>MGDCDIEGKDGKQYESVLMVSIDQLLDSMKEIGSNCLNNEFNFFKRHICDANKE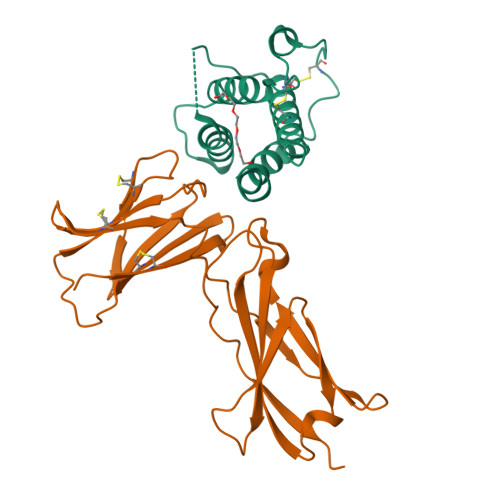GMFLFRAARKLRQFLKMNSTGDFDLHLLKVSEGTTILLNCTGQVKGRKPAALGAAQPTKSLEENKSLKEQKKLNDLCFLKRLLQEIKTCWNKILMGTKEH[2x];>GSHMESGYAQNGDLEDAELDDYSFSCYSQLEVNGSQHSLTCAFEDPDVNTTNLEFEICGALVEVKCLNFRKLQEIYFIETKKFLLIGKSNICVKVGEKSLTCKKIDLTTIVKPEAPFDLSVVYREGANDFVVTFNTSHLQKKYVKVLMHDVAYRQEKDENKWTHVNLSSTKLTLLQRKLQPAAMYEIKVRSIPDHYFKGFWSEWSPSYYFRTPEINNSSGEMD[2x]>[6x]SVIKPDMKIKLRMEGAVNGHPFAIEGVGLGKPFEGKQSMDLKVKEGGPLPFAYDILTMAFCYGNRVFAKYPENIVDYFKQSFPEGYSWERSMIYEDGGICNATNDITLD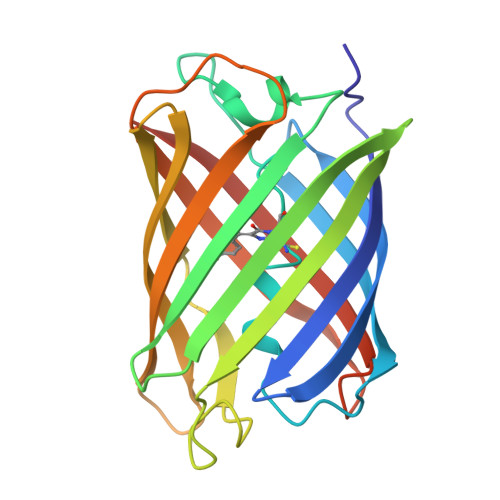GDCYIYEIRFDGVNFPANGPVMQKRTVKWELSTEKLYVRDGVLKSDGNYALSLEGGGHYRCDFKTTYKAKKVVQLPDYHSVDHHIEIKSHDKDYSNVNLHEHAEAHSELPRQAK> MKEKIFNELTRKMKRKEISAKIQREENKQILIRQRNNKKYIQSIQGIQQERKKGKLYLVEMATQNVEEMDTIQKMNY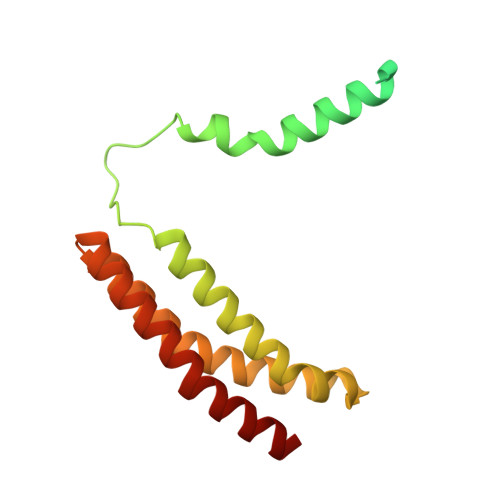EATVNMGRQDLITREYTFYSDYEFIPIQEDRKQQMEDALNNLHKIIHPTVTQLKKKANVQEIQDRVFRKLQGWEGELNTCVFSAKNVRDSNFCADRFTNRINTEGVEFVKQILREY> UCGC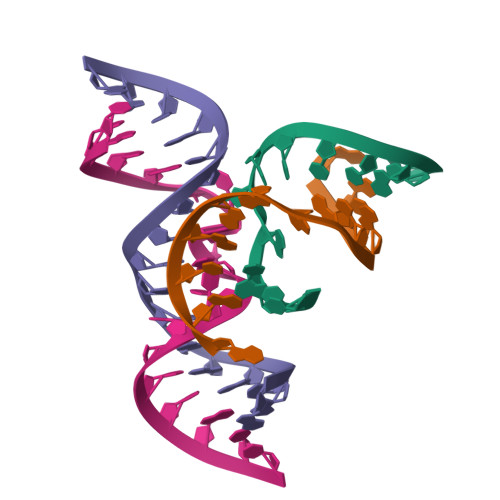AGUCCUAUU;> AAUAGAGAAGCGA;> GGCAGAGAAACACACGA;> UCGUGGUACAUUACCUGCC>MFVALGAQIYRQYFGRRGMAMANNSSVANKVCLIVIDGWGVSEDPYGNAILNAQTPVMDKLCSGNWAQIEAHGLHVGLPEGLMGNSEVGHLNIGAGRVIYQDIVRINLAVKNNKFVTNESLVDACDRAKNGNGRLHLAGLVSDGGVHSHIDHMFALVKAIKELGVPELYLHFYGDGRDTSPNSGVGFLEQTLEFLEKTTGYGKLATVVGRYYAMDRDNRWERINVAYEAMIGGVGETSDEAGVVEVVRKRYAADETDEFLKPIILQGEKGRVQNDDTIIFFDYRADRMREISAAMGMDRYKDCNSKLAHPSNLQVYGMTQYKAEFPFKSLFPPASNKNVLAEWLAEQKVSQFHCAETEKYAHVTFFFNGGLEKQFEGEERCLVPSPKVATYDLQPEMSAAGVADKMIEQLEAGTHPFIMCNFAPPDMVGHTGVYEAAVKACEATDIAIGRIYEATQKHGYSLMVTADHGNAEKMKAPDGGKHTAHTCYRVPLTLSHPGFKFVDPADRHPALCDVAPTVLAIMGLPQPAEMTGVSIVQKIKLAAALEHHHHHH[2x]

Phosphoglycerate mutases (PGMs) catalyse the interconversion of 2- and 3-phosphoglycerate (2-PG; 3-PG) in the glycolytic and gluconeogenic pathways. The enzymes have no amino-acid sequence similarity and differ in their mechanism of catalysis. iPGM is comprised of ∼510 amino acids and facilitates the intramolecular transfer of the phosphoryl group on the monophosphoglycerates through a phosphoserine intermediate and is the sole PGM in nematode. The iPGMs are monomeric bi-domain enzymes where a phosphatase domain, structurally related to the alkaline phosphatase family of binuclear metalloenzymes, is connected by two hinge peptides to a phosphotransferase domain8. The glycolytic phosphoglycerate mutase, iPGM is an attractive target for the development of broad spectrum antiparasitic and antibacterial agents owing to its essential metabolic function and evolutionary divergence from the human enzyme.

Although soaking of pre-formed iPGM crystals with Ce-2 caused the crystals to shatter, we succeeded in obtaining two apo crystal forms, monoclinic P (iPGM-m) and orthorhombic P (iPGM-o) lattices of native C. elegans iPGM. These crystals provided the structure of a nematode iPGM. As anticipated from primary amino-acid sequence homology among iPGM orthologues, C. elegans iPGM is quite similar to other iPGMs of bacterial origin. Similar to other iPGMs, Mn2+ occupies one of the two phosphatase domain metal ion binding sites while, as in alkaline phosphatase, a Zn2+ ion was found in the second binding site of C. elegans iPGM. The identity of these transition metal ions was verified from phased anomalous difference maps calculated from data collected at wavelengths of 1.0000 and 1.9016 Å. These metal ions contact the histidine and aspartate triads as shown in Supplementary Fig. 12 at coordination distances listed in Supplementary Table 6, and the catalytic Ser86 nucleophile coordinates to the Zn2+ ion. From the apo iPGM structure we observed that the N-terminal 18 amino acids, unique to C. elegans iPGM, were disordered.>MHKLLLALLSLSLVGCIDSKEEILEEKNQGLVYCAEANPVSFNPQVTTTGSTIDIIANQLYDRLISIDPVTAEFKSELATDWKISKDGKSVTFTLRKGVKFHT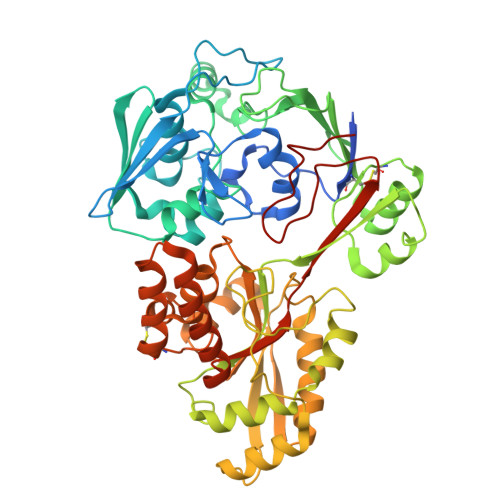TAYFTPTREFNADDVIFTFSRLFDVYNPYHFVGDANYPYFQSVGIDQLIRKIVRVSDHQVRFELFNAESSFLANMATDFAVVLSKEYAMALKANNQENLFDQYPVGTGPYIYKEYRRDHLVRFYKNADYWKHEVALEQLVYDITPNGTTRIAKILTKECDVTAHPSSAQLSILAQRDDINVERETNLNIGYWAFNTERPPFDNLKVRQALVHAIDIEKIMQAVYYGNGLRARSILPPTSWAFEPQKNMPIFDPQLAKKLLTEAGYEKGFDMSIWAMPVSRIYNPNARKMAELMQSDLRKIGVNVNIVEYEWNTFIQRIGEHRHDSVLLGWAADTPDPDNFFSPLLSCTATFSGKNPANWCNPEFDLLLTKALDTTDLNLRKQYYDAAQSMIIEQLPLYPIAHGMRFQASSADVEGITLGPFGAISLANARKKHHHHHH[8x]> HHHHHHMPFTLGQRWISDTESELGLGTVVAVDARTVTLLFPSTGENRLYARSDSPVTRVMFNPGDTITSHDGWQMQVEEVKEENGLLTYIGTRLDTEESGVALREVFLDSKLVFSKPQDRLFAGQIDRMDRFALRYRARKYSSEQFRMPYSGLRGQRTSLIPHQLNIAHDVGRRHAPRVLLADEVGLGKTIEAGMILHQQLLSGAAERVLIIVPETLQHQWLVEMLRRFNLRFALFDDERYAEAQHDAYNPFDTEQLVICSLDFARRSKQRLEHLCEAEWDLLVVDEAHHLVWSEDAPSREYQAIEQLAEHVPGVLLLTATPEQLGMESHFARLRLLDPNRFHDFAQFVEEQKNYCPVADAVAMLLAGNKLSNDELNMLGEMIGEQDIEPLLQAANSDSEDAQSARQELVSMLMDRHGTSRVLFRNTRNGVKGFPKRELHTIKLPLPTQYQTAIKVSGIMGARKSAEDRARDMLYPERIYQEFEGDNATWWNFDPRVEWLMGYLTSHRSQKVLVICAKAATALQLE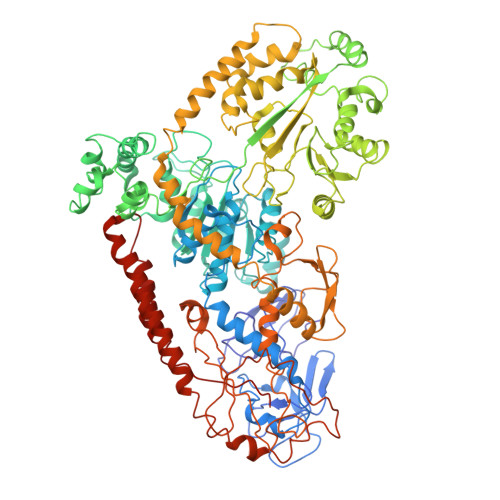QVLREREGIRAAVFHEGMSIIERDRAAAWFAEEDTGAQVLLCSEIGSEGRNFQFASHMVMFDLPFNPDLLEQRIGRLDRIGQAHDIQIHVPYLEKTAQSVLVRWYHEGLDAFEHTCPTGRTIYDSVYNDLINYLASPDQTEGFDDLIKNCREQHEALKAQLEQGRDRLLEIHSNGGEKAQALAESIEEQDDDTNLIAFAMNLFDIIGINQDDRGDNMIVLTPSDHMLVPDFPGLSEDGITITFDREVALAREDAQFITWEHPLIRNGLDLILSGDTGSSTISLLKNKALPVGTLLVELIYVVEAQAPKQLQLNRFLPPTPVRMLLDKNGNNLAAQVEFETFNRQLNAVNRHTGSKLVNAVQQDVHAILQLGEAQIEKSARALIDAARNEADEKLSAELSRLEALRAVNPNIRDDELTAIESNRQQVMESLDQAGWRLDALRLIVVTHQ>XPPGPPGPTGPRGPPGPPGX[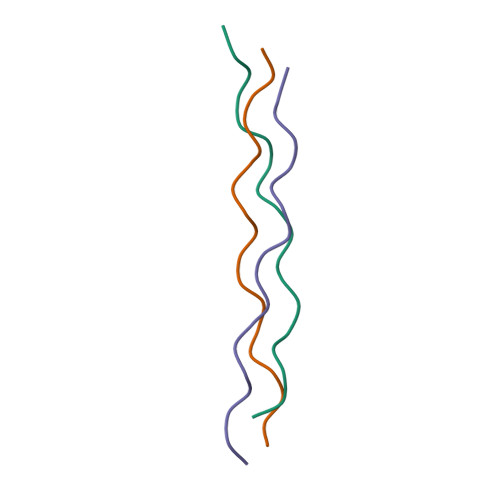3x]> GPMQPRLKVGAIPDQNPERLNRLYGQLADELSDRLNVKVRYVPVSNYPAAVSAFRTGGLDLVWFGGLTGVQARLQTPGAQVLAQRDIDARFRSVFIANTSSGLQPISSINGLTSLRGKRFSFGSESSTSGRLMPQHFLAKAGVTPSQFSGGRAGFSGSHDATIAVVQSGAYEAGALNEQVWTSAVNDGRVNTEKVSVIWRTPEYVDYHWVVRPKLDQRFGKGFTTRLQKA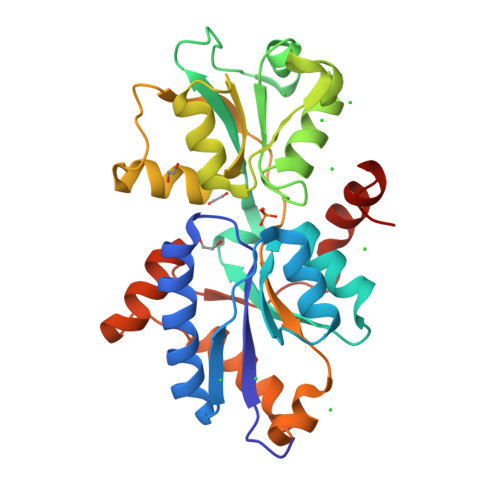ILGLEPTTPRQVTILELFAAKRFIPVEASQYKPIEKVGRELGKIR>[8x]GMEPFKQQKVEDFYDIGEELGSGQFAIVKKCREKSTGLEYAAKFIKKRQSRASRRGVSREEIEREVSILRQVLHHNVI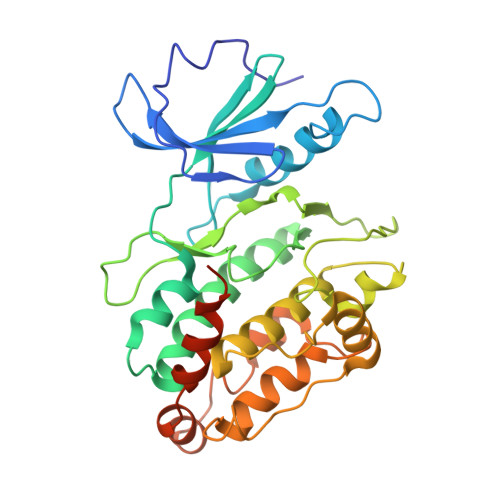TLHDVYENRTDVVLILELVSGGELFDFLAQKESLSEEEATSFIKQILDGVNYLHTKKIAHFDLKPENIMLLDKNIPIPHIKLIDFGLAHEIEDGVEFKNIFGTPEFVAPEIVNYEPLGLEADMWSIGVITYILLSGASPFLGDTKQETLANITAVSYDFDEEFFSQTSELAKDFIRKLLVKETRKRLTIQEALRHPWITPVDNQQAMVRRESVVNLENFRKQYVRRRWKLDFSIVSLCNHLTR> MPIDRKTLCHLLSVLPLALLGSHVARASTPGIVIPPQEQITQHGSPYGRCANKTRALTVAELRGSG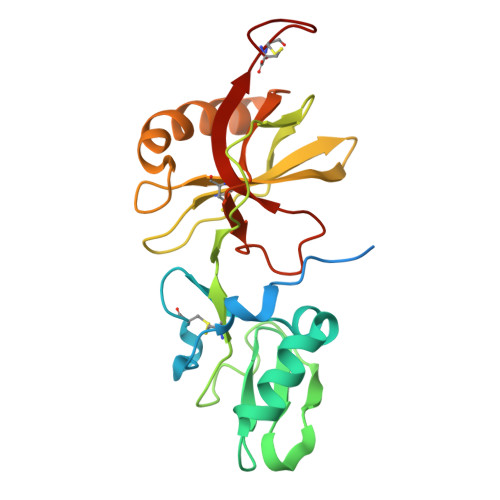DLQEYLRHVTRGWSIFALYDGTYLGGEYGGVIKDGTPGGAFDLKTTFCIMTTRNTGQPATDHYYSNVTATRLLSSTNSRLCAVFVRSGQPVIGACTSPYDGKYWSMYSRLRKMLYLIYVAGISVRVHVSKEEQYYDYEDATFETYALTGISICNPGSSLC> AKMAFTLADRVTEEMLADKAALVVEVVEENYHDAPIVGIAVVNEHGRFFLRPETALADPQFVAWLGDETKKKSMFDSKRAAVALKWKGIELCGVSFDLLLAAYLLDPAQGVDDVAAAAKMKQYEAVRPDEAVYGKGAKRAVPDEPVLAEHLVRKAA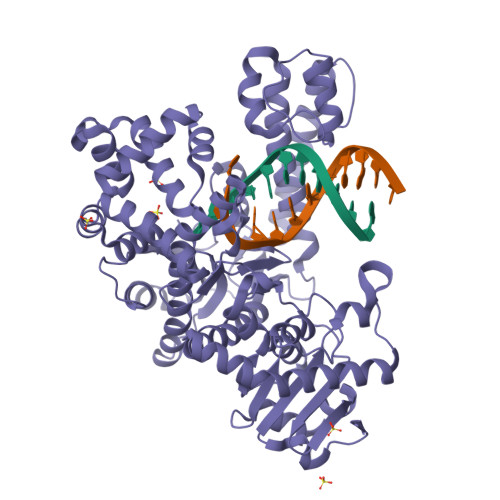AIWALERPFLDELRRNEQDRLLVELEQPLSSILAEMEFAGVKVDTKRLEQMGEELAEQLRTVEQRIYELAGQEFNINSPKQLGVILFEKLQLPVLKKTKTGYSTSADVLEKLAPYHEIVENILHYRQLGKLQSTYIEGLLKVVRPDTKKVHTIFNQALTQTGRLSSTEPNLQNIPIRLEEGRKIRQAFVPSESDWLIFAADYSQIELRVLAHIAEDDNLMEAFRRDLDIHTKTAMDIFQVSEDEVTPNMRRQAKAVNFGIVYGISDYGLAQNLNISRKEAAEFIERYFESFPGVKRYMENIVQEAKQKGYVTTLLHRRRYLPDITSRNFNVRSFAERMAMNTPIQGSAADIIKKAMIDLNARLKEERLQARLLLQVHDELILEAPKEEMERLCRLVPEVMEQAVTLRVPLKVDYHYGSTWYDAK>[6x]MKENKLDYIPEPMDLSLVDLPESLIQLSERIAENVHEVWAKA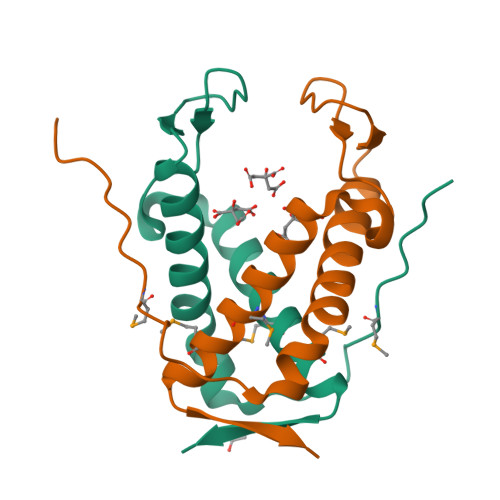RIDEGWTYGEKRDDIHKKHPCLVPYDELPEEEKEADRNTAMNTIKMVKKLGFRIEKED> RSKS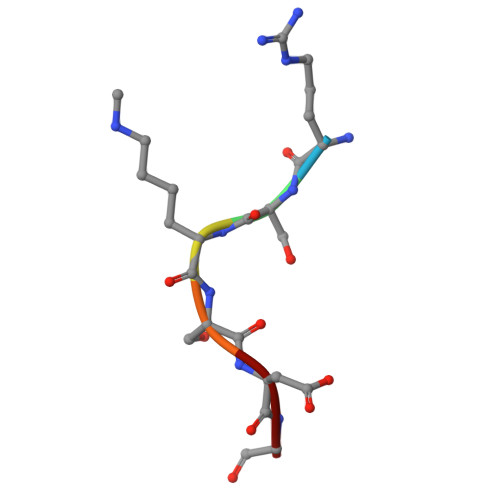DG>MGHHHHHHMSPNLPGQTTVQVRVPYRVVGLVVGPKGATIKRIQQQTHTYIVTPSRDKEPVFEVTGMPENVDR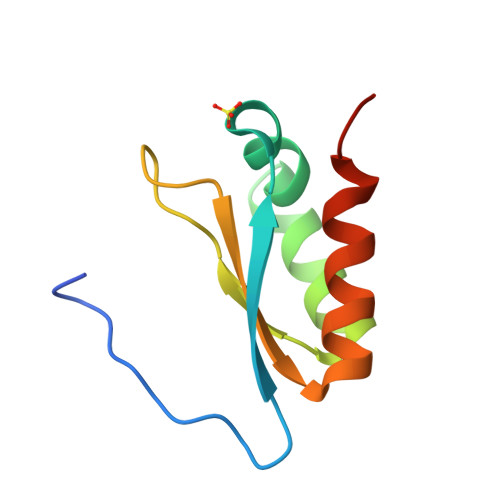AREEIEMHIAMRTG[3x]> MRCIGISNRDFVEGVSGGSWVDIVLEHGSCVTTMAKNKPTLDFELIKTEAKQPATLRKYCIEAKLTNTTTESRCPTQGEPTLNEEQDKRFVCKHSMVDRGWGNGCGLFGKGGIVTCAMFTCKKNMEGKIVQPENLEYTVVITPHSGEEHAVGNDTGKHGKEVKITPQSSITEAELTGYGTVTMECSPRTGLDFNEMVLLQMKDKAWLVHRQWFLDLPLPWLPGADTQGSNWIQKETLVTFKNPHAKKQDVVVLGSQEGAMHTALTGATEIQMSSGNLLFTGHLKCRLRMDKLQLKGMSYSMCTGKFKVVKEIAETQHGTIVIRVQYEGDGSPCKIPFEIMDLE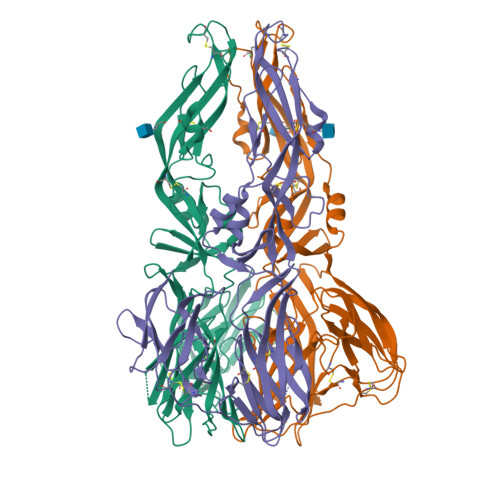KRHVLGRLITVNPIVTEKDSPVNIEAEPPFGDSYIIIGVEPGQLKLNWFKK>[28x]HHHHHHENLYFQGMSFDNYLVPTVIEQSGRGERAFDIYSRLLKARIVFL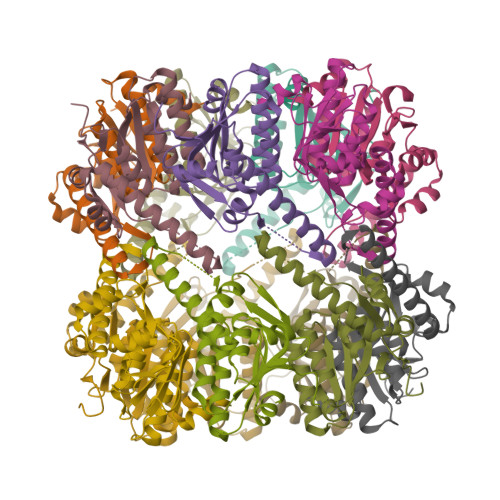VGPVTDESANLVVAQLLFLESANPDKDIFFYINSPGGSVTAGMSIYDTMNFIKPDVSTLCLGQAASMGAFLLSAGEKGKRFALPNSRIMIHQPLISGGLGGQASDIEIHARELLKIKEKLNRLMAKHCDRDLADLERDTDRDNFMSAEEAKEYGLIDQILENRASLRL>[2x]MGSSHHHHHHSSGLVPRGSHMTAPGHTSVQTPIAGLVELALSDPSLQDVIRRAADRPADLALVGPASARVLVAAALAQNGPLLVVAATGREADELTAELRGVFGDSVALFPSWETLPHERLSPGVETVGARLMLLRRLARPDDETLGAPLRVVVTTTRSLLQPMAPDLVDIEPVTLSVGAEMEFEDVVARLVDLSYTRVDMVGKRGEFAVRGGILDVFPPTAEHPVRVEFWGDEISEMRAFAIADQRSIPEVPVQTVVAVPCRELLMTDDVRERAAALAAEHPTTENTVPGTVPDMLAKLAEGIPVDGMEALLPLLHPIEPTTLTRHLPEGAPVLVCDPEKVRTRAADLIKTGREFLEASWSTAAVGGDAPIDLEALGASGFVTFEEAREAAREGGHPWWTLSQLSDESAVELDIRSAPSARGSQHNLEEIFAMLRAHVATGGYAAVVTPGIGTAHRVVEQLGEADTAATILEPGTAPKAGVVGVLKGPLCSGVVLPGANLVIITETD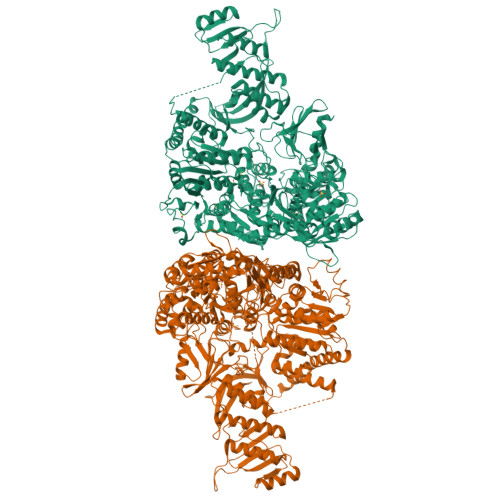LTGNRVTANEGRKLAAKRRNVVDPLALTAGDLVVHDQHGIGKFVEMTERVVGGARREYLVLEYASSKRGGGTDKLYVPMDSLDQLSRYVGGEAPSLSRLGGSDWANTKTKARRAVREIASELVALYAKRQSAPGHAFGPDTPWQAEMEDAFGFTETIDQLTAIQEVKSDMEKPVPMDRVICGDVGYGKTEIAVRAAFKAVQDGKQVAVLVPTTLLADQHLQTFTNRMAGFPVTVKGLSRFTDPAESRAVIEGLKDGSVDVVIGTHRLLQTGVTWKDLGLIIVDEEQRFGVEHKEHIKSMRTHVDVLTMSATPIPRTLEMSLAGIREMSTILTPPEERYPVLTYVGPHDDKQVAAALRRELLRDGQAFYIHNRVRTIDEAAARVRQLVPEARVVVAHGQMNEETLEKTVEGFWNREYDILVCTTIVETGLDISNANTLIVERADTFGLSQLHQLRGRVGRSRERGYAYFLYPPNKPLTETAYDRLATIAQNNELGAGMAVAMKDLEIRGAGNVLGAEQSGHVAGVGFDLYVRLVGEAVEAYRAAADGKTVATPQEQKDVRIDLPVDAHLPPEYIGSDRLRLEAYRRLAAAADDDAVASVVDELIDRYGPLPEPAQRLVAVARLRLLCREFGITEIGAVSASTVRLSPMVLPDSAQLRLKRMYPGGHYRATTSTVQVPLPRAGEGVGAPRIRDLELVQWVAGLVLVLNGKGQGDVDMSKFSNPAGEAKR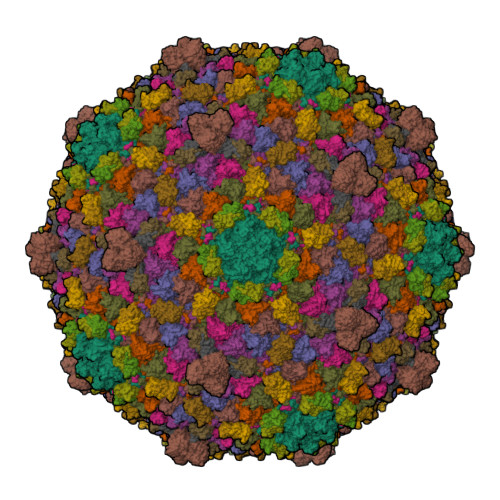>[7x]MALNNTTYQGSMRGYAVTKSRLDSFIPEVWTGEVLRALNQNFVASQYVKTLDVTGKKGDRFHIPNIGRASVFDKLPETPVQLQARQESDFYVDIDKYKESSFLIEDLGAMQSSYDIRQEYTTEAGYALSRMMDADILGLRAAVKGLNNGSEIFNTADATISGASSPLNYQALLTAKTILDNRDVPMEKRVIITSPTGYNQLLAIDKFISMDYQDGRPVKSGVVGTIFGIPVIMTTQVTVNSATGYSNGSTVTGIPTPGVSGAGALHLPTQDVFTSLPTAFTGANTGLAAQVITTLMCHSDWAVMLKSKMPSAESDRSVQYLGDIVVNSMVYGAKLFRQTNAVIINHNAVIPAVV;> MSIAWYRELYGTEPNFNYPNGVLVPNHPGYNQTPGGIYLPNVAALSGAAITANRIHYVYFQVAQTFVTDALVFRVSTAVTGNARVGLYTVDPSSGFPQFLVTQGSAAALTGGSTGDRVVLINRGIVTLPPTWYMTAIVSDVAANLAGINGSATAQYYRQPSIPSGGSGCYTAPFTYGVLPDLAPTPDAVSTTNHPVVGLRTA;>[7x]MAITCTACTFTMTDAEFAILNEGVAAPTIDPRGSFAGLQSLSGAPITASASAGTTTVVVAASNRNDANIRTLAQRLRRAAQANRITFTA> GSHMTWLSDFPQAWAETGGMGLAVRQAPLIIPLKATSTPVSIKQYPMSQEARLGIKPHIQRLLDQGILVPCQSPWNTPLLPVKKPGTNDYRPVQDLREVNKRVEDIHPTVPNPYNLLSGLPPSHQWYTVLDLKDAFFCLRLHPTSQPLFAFEWRDPEMGISGQLTWTRLPQGFKNSPTLFDEALHRDLADFRIQHPDLILLQYVDDLLLAATSELDCQQGTRALLQTLGNLGYRASAKKAQICQKQVKYLGYLLKEGQRLTRGSGC

Using a host–guest system in which Moloney murine leukemia virus reverse transcriptase serves as the host and DNA as the guests, we determined high-resolution crystal structures of three complexes including 5′-CTTBPPBBSSZZSAAG, 5′-CTTSSPBZPSZBBAAG and 5′-CTTZZPBSBSZPPAAG with 10 consecutive unnatural nucleobase pairs in B-form within self-complementary 16 bp duplex oligonucleotides. We refer to this ALternative Isoinformational ENgineered (ALIEN) genetic system containing two nucleobase pairs (P:Z, pairing 2-amino-imidazo-[1,2-a]-1,3,5-triazin-(8H)-4-one with 6-amino-5-nitro-(1H)-pyridin-2-one, and B:S, 6-amino-4-hydroxy-5-(1H)-purin-2-one with 3-methyl-6-amino-pyrimidin-2-one) as ALIEN DNA. Three hydrogen bonds that join the P:Z and B:S pairs are stereochemically distinct from each other and from those of standard nucleobase pairs. Interactions between the protein and DNA are limited to hydrogen-bonding interactions of Arg 116 with the minor groove of the terminal base pairs within the duplex, leaving the remainder of the duplex free to adopt its preferred sequence-specific structure.

The BPPBB structure includes a tract with five consecutive purines (or five pyrimidines on the complementary strand), offering the first view of a purine-rich tract in ALIEN DNA. Superpositioning of the ALIEN DNA in the host–guest structures results in r.m.s.d. values ranging from 0.6 to 2.6 Å, with the most similar being SSPBZ and SZZPBS and the least similar being BPPBB and ZZPBS. It is not surprising that BPPBB differs from the other structures, since it contains five consecutive purine nucleobases; the other structures exhibit a pattern of two pyrimidine, two purine and a pyrimidine. In the BPPBB structure, the B:S pair at position 4 forms only two hydrogen bonds between O2 of B and N2 of S, N1 of B and N3 of S. The second BPPBB point that falls outside the B cluster is the BS/BS step (positions 8 and 9). For slide versus roll, two points fall in the same quadrants of the graph as B-DNA but extend beyond these values; these points are the SP/ZB point for the SSPBZ structure, in which the slide value is 3.03 Å, and the BS/BS point for the BPPBB structure, with a slide value of 2.81 Å and a roll value of −21.52°. However, the value of the BS/BS step (position 8 and 9) of BPPBB falls out of the range, with an x-displacement of 4.73 Å and inclination value of −26.46°. BS/BS (positions 8 and 9) in the BPPBB structure has a slide value of 2.8 Å, and the SP/ZB step in the SSPBZ structure a value of 3.0 Å. The same dinucleotide step, BS/BS in the BPPBB structure, has a roll angle of −21.5°. The range for roll angles in natural DNA is −10° to 11.7°. This is likely a consequence of the five consecutive purine nucleobases abutting five consecutive pyrimidines across the central dyad of the oligonucleotide. The BPPBB structure has a slide value of 2.8 Å at step position 8, a feature distinguishing it from the other structures.> MKKWLITSGVVFSLFSTSSFAVMGKRYVATPQQSQWEMVVNTPLECQLVHPIPSFGDAVFSSRANKKINLDFELKMRRPMGETRNVSLISMPPPWRPGEHADRITNLKFFKQFDGYVGGQTAWGILSELEKGRYPTFSYQDWQSRDQRIEVALSSVLFQNKYNAFSDCISNLLKYSFEDIAFTILHYERQGDQLTKASKKRLSQIADYIRHNQDIDLVLVATYTDSTDGKSASQS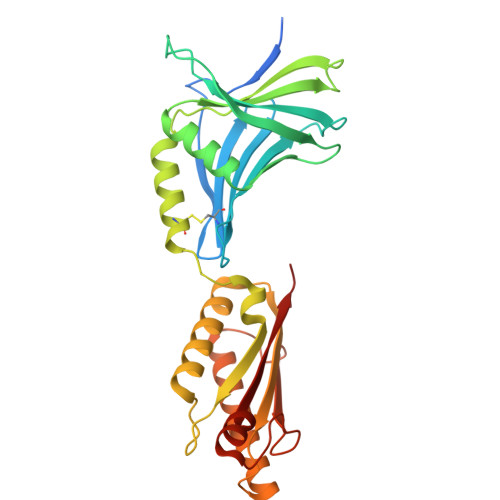LSERRAESLRDYFQSLGLPEDRIQVQGYGKRRPIADNGSPIGKDKNRRVVISLGRTQV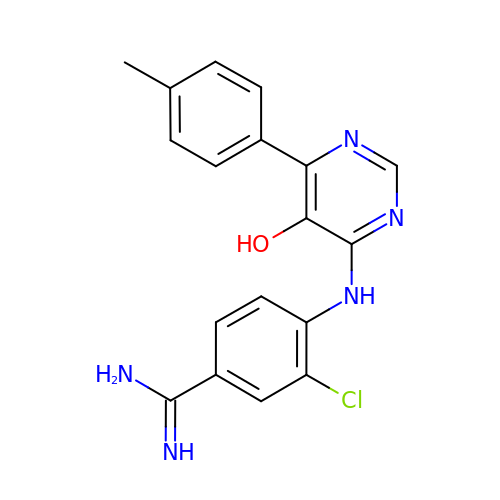3-chloro-4-{[5-hydroxy-6-(4-methylphenyl)pyrimidin-4-yl]amino}benzene-1-carboximidamide | C18 H16 Cl N5 O | SNGWZJUYWHIFIM-UHFFFAOYSA-N> GNYNVF

The protein hnRNPA2 functions in RNA stabilization, splicing, trafficking, and translation. In its role in protecting mRNAs, it is a component of cytoplasmic stress granules, one of the so-called membraneless organelles (MLOs). Its 341 amino-acid-residue sequence contains an RNA-binding domain (RBD) with two RNA recognition motifs (RRMs) and a 161-residue C-terminal low-complexity domain (LCD). The LCD is rich in Gly, Tyr, Phe, Asn, and Asp residues, and poor in hydrophobes, with Val, Ala, Leu, and Ile entirely absent.

A missense point mutation that converts a conserved aspartic acid to a valine (D290V) in hnRNPA2-LCD was identified in 2013 as being associated with ALS and MSP2. To investigate the structural differences between the wildtype and the mutant, we crystallized the hexamer segment 286GNYNVF291 containing the disease-causing mutation and determined its structure by X-ray crystallography (Fig. 4a and Statistics in Table 3). As expected, the crystal structure of the mutant segment forms a steric zipper motif and the sidechains of the two β-sheets mate tightly with each other in a dry interface. The area buried (Ab) and shape complementarity (Sc) for the mutant segment are 104 Å2 per chain and 0.86, respectively. The mutant segment structure forms in-register, parallel β-sheets. The backbones of the wildtype structure and the mutant segment fit well with each other, whereas the sidechain of Asp290 in the wildtype structure clashes with Asn289 of the mating sheet of mutant steric zipper, disrupting the steric zipper formation. When the conserved Asp290 residue is mutated to a Val, the mutation enables a more stable steric zipper interaction that was previously prevented by the Asp290 sidechain. The mutant segment, as we expected, precipitated after shaking (left), and TEM images showed that the precipitates were composed of micro-crystals (left). The results suggest that the mutant segment with the pathogenic mutation forms a more stable structure than the WT segment, and converts a gel-promoting segment into an aggregation-promoting segment. Unsurprisingly, the mutant segment is an outlier in terms of having greater energetic stability than any hexameric segment in either hnRNPA2 or FUS.> MVAEKETLSLNKCPDKMPKRTKLLAQQPLPVHQPHSLVSEGFTVKAMMKNSVVRGPPAAGAFKERPTKPTAFRKFYERGDFPIALEHDSKGNKIAWKVEI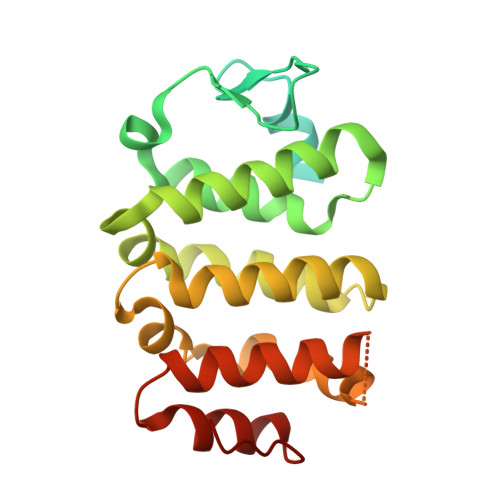EKLDYHHYLPLFFDGLCEMTFPYEFFARQGIHDMLEHGGNKILPVLPQLIIPIKNALNLRNRQVICVTLKVLQHLVVSAEMVGKALVPYYRQILPVLNIFKNMNVNSGDGIDYSQQKRENIGDLIQETLEAFERYGGENAFINIKYVVPTYESCLLN>MDFSKMSIVGRIGSEFTEHTSANNNRYLKYSIASQPRRDGQTNWYNITVFNEPQINFLTEYVRKGALVYVEADAANYVFERDDGSKGTTLSL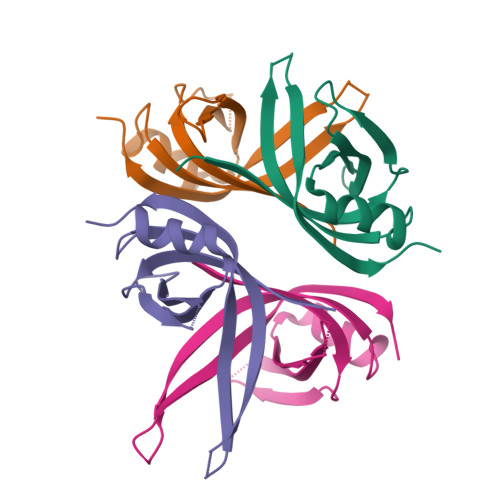VQKDINLLKNGKKLEDAEGQENAASSE[8x]> MAHHHHHHMILCCGEALIDMLPRETTGGETAFQPFAGGSVFNTAIALGRLGVPTGFFSGISSDFFGDVLRDTLARSNVDYSFAAISNRPTTLAFVRLVDGQARYA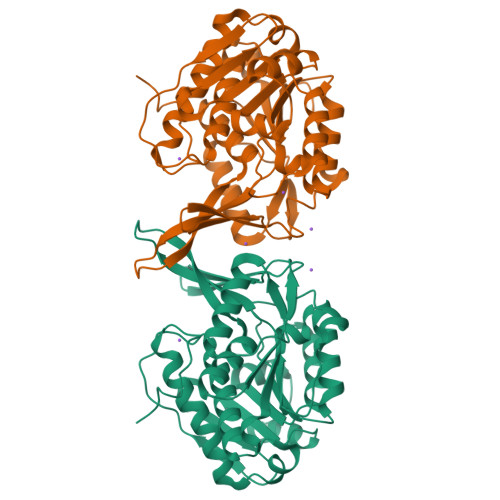FYDENTAGRMLSRNDMPYVDETISAMLFGCISLISEPCGSVYETLLAREAPNRVMFLDPNIRANLITVRKTHLTRMKRMIALADIVKLSDEDLDWFGEKGSHDEIAAEWLKLGPKLVVITKGAHGAVAYTNHATVPVPGVKVDVVDTVGAGDTVNAGILASLHSQGLLTKDALANLSEDQIHSAVALGVRAAAVTVSRAGANPPWAHEMRD N-(2-(((5-CHLORO-2-PYRIDINYL)AMINO)SULFONYL)PHENYL)-4-(2-OXO-1(2H)-PYRIDINYL)BENZAMIDE | C23 H17 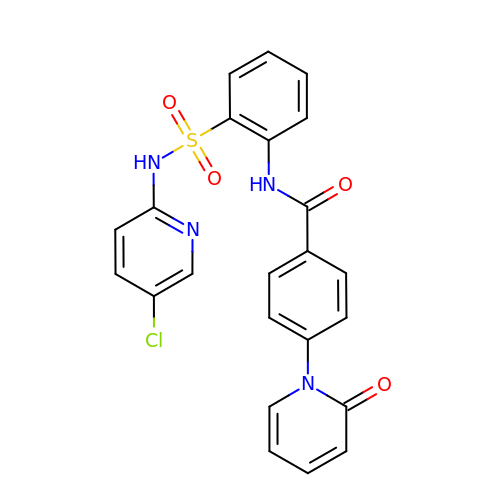Cl N4 O4 S | MIJGLXFQYBTIFY-UHFFFAOYSA-N>MGSSHHHHHHSQDPIRRGDVYLADLSPVQGSEQGGVRPVVIIQNDTGNKYSPTVIVAAITGRINKAKIPTHVEIEKKKYKLDKDSVILLEQIRTLDKKRLKEKLTYLSDDKMKEVDNALMISLGLNAVAHQKN[8x]

TA modules are small operons encoding two proteins: a ‘toxin’ that interferes with basic cellular metabolism, usually translation or transcription, and an ‘antitoxin’ that neutralizes the toxin and protects the cell from its potentially destructive activity (for reviews see 1–4). The toxin MazF is activated under a number of stressful conditions via proteolytic degradation of its neutralizing antitoxin MazE by the ClpPA or Lon proteases, (18,30,35) and was proposed to be under control of quorum sensing. In this paper, we present a method to obtain large quantities of active SaMazF and provide the structure of this protein as determined by nuclear magnetic resonance (NMR) and X-ray crystallography. The SaMazF dimer is formed by pairing strand S6 from two monomers to form a dimer-wide 10-strand anti-parallel β-sheet.

Three different crystal forms of SaMazF are available, which lead to the structures of 14 crystallographically independent SaMazF monomers forming 7 independent dimers. Each of these monomers was independently refined except for the eight monomers present in crystal form III, which were restrained by NCS because of the lower resolution (excluding two more variable loops that clearly adopt distinct conformations). Overall, the structures of the SaMazF monomers are very similar with pair-wise backbone root-mean-square deviations (RMSDs) of 0.18–0.58 Å for all 99 residues defined in each molecule (the 8 NCS restrained monomers from crystal form III are represented in this comparison by chain A only). Loop S4-S5 (Ile61-Lys70) is involved in lattice contacts in most but not all SaMazF monomers. Four classes of conformations are observed. The most common conformation is observed in ten chains, two cases of which do not involve lattice contacts. In the remaining four chains, this conformation is prohibited as it would lead to steric clashes with a neighboring monomer. Of these remaining chains, form II chains A and B adopt the same conformation while form III chains D and E each adopt a unique conformation. Loops S4-S5 of the latter four chains are all involved in lattice contacts. Thus, it seems like loop S4-S5 will adopt a default conformation when the crystal environment allows for it, but will adapt its conformation otherwise.>[4x]MAGKEIQTPDQAEAFVAKVFDVLDSYDYTRFGEVLSTDLKYEGGLQKTSGLDNFINDIKASTQRMPGLQTSHSRYRTELTAEGTIYSEGHSNASLESNPGKVVTVPM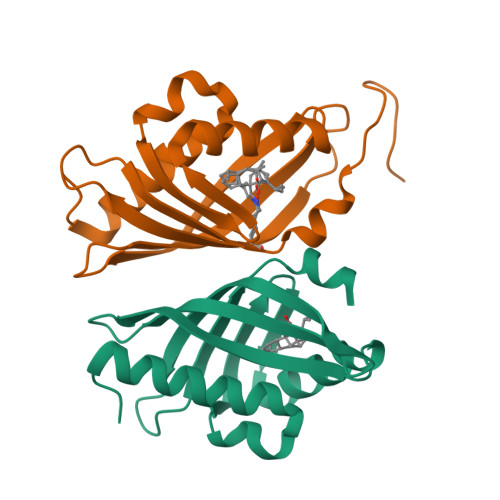IGVFKLDSEDGKIKEMRIYKDRLPFLALHQALPGMKANN Contrary to most organisms in which three enzymes compose the 2-oxoglutarate dehydrogenase complex (ODH), actinobacteria rely on a two-in-one protein (OdhA) in which both the oxidative decarboxylation and succinyl transferase steps are carried out by the same polypeptide. Here we describe high-resolution cryo-EM and crystallographic snapshots of representative enzymes from Mycobacterium smegmatis and Corynebacterium glutamicum, showing that OdhA is an 800-kDa homohexamer that assembles into a three-blade propeller shape. The obligate trimeric and dimeric states of the acyltransferase and dehydrogenase domains, respectively, are critical for maintaining the overall assembly, where both domains interact via subtle readjustments of their interfaces. Schematic illustration of the reaction steps involved in the oxidative decarboxylation of 2-oxoglutarate with generation of succinyl-CoA and NADH/H+ (ODH reaction), with emphasis on the catalytic steps catalyzed by OdhA. These include the ThDP-dependent decarboxylation of the 2-oxoglutarate substrate followed the reductive acylation of the lipoyl group provided by E2p (both catalyzed by the OdhA E1o domain), and the transfer of the succinyl moiety to the CoASH acceptor (catalyzed by the OdhA E2o domain).

Therefore, based on the MsKGD structure and on secondary structure predictions, we produced a truncated version of OdhA deprived of the flexible N-terminal segment (OdhAΔ97), which produced crystals diffracting up to 2.5 Å resolution. The single protomer shows the presence of an N-terminal acyltransferase (E2o) domain, spanning from the construct N-terminus to residue Asn349, connected by a 17-residue linker to the C-terminal, ThDP-dependent oxoglutarate dehydrogenase domain (E1o). In addition, a ThDP-Mg2+ cofactor is bound at the E1o domain dimeric interface, in an equivalent pose and active site environment as in the M. smegmatis E1o (MsKGDΔ360) high-resolution crystal structures. On the other hand, the E2o N-terminal domain shows the known, compact triangular trimeric conformation of the chloramphenicol acetyltransferase (CAT) family, characterized by an N-terminal β-strand that protrudes to make a strand exchange (mixed β-sheet) with the neighboring monomer. Furthermore, despite the overall conservation of the CAT fold, a notable difference between the OdhA succinyltransferase domain and other E2o domains resides in the β-harpin that normally lies close to the three-fold axis and is located on the inside surface of the cubic assembly, here replaced by a short α-helix (connected by flexible linkers) spanning residues 296-302.

> GKLPEPGQTPIRGIFKSIAKNMDISLEIPTATSVRDMPARLMFENRAMVNDQLKRTRGGKISFTHIIGYAMVKAVMAHPDMNNSYDVIDGKPTLIVPEHINLGLAIDLPQKDGSRALVVAAIKETEKMNFSEFLAAYEDIVARSRKGKLTMDDYQGVTVSLTNPGGIGTRHSVPRLTKGQGTIIGVGSMDYPAEFQGASEDRLAELGVGKLVTITSTYDHRVIQGAVSGEFLRTMSRLLTDDSFWDEIFDAMNVPYTPMRWAQDVPNTGVDKNTRVMQLIEAYRSRGHLIADTNPLSWVQPGMPVPDHRDLDIETHNLTIWDLDRTFNVGGFGGKETMTLREVLSRLRAAYTLKVGSEYTHILDRDERTWLQDRLEAGMPKPTQAEQKYILQKLNAAEAFENFLQTKYVGQKRFSLEGAEALIPLMDSAIDTAAGQGLDEVVIGMPHRGRLNVLFNIVGKPLASIFNEFEGQMEQGQIGGSGDVKYHLGSEGQHLQMFGDGEIKVSLTANPSHLEAVNPVMEGIVRAKQDYLDKGVDGKTVVPLLLHGDAAFAGLGIVPETINLAKLRGYDVGGTIHIVVNNQIGFTTTPDSSRSMHYATDYAKAFGCPVFHVNGDDPEAVVWVGQLATEYRRRFGKDVFIDLVCYRLRGHNEADDPSMTQPKMYELITGRETVRAQYTEDLLGRGDLSNEDAEAVVRDFHDQMESVFNEVKEGGKKQAEAQTGITGSQKLPHGLETNISREELLELGQAFANTPEGFNYHPRVAPVAKKRVSSVTEGGIDWAWGELLAFGSLANSGRLVRLAGEDSRRGTFTQRHAVAIDPATAEEFNPLHELAQSKGNNGKFLVYNSALTEYAGMGFEYGYSVGNEDSIVAWEAQFGDFANGAQTIIDEYVSSGEAKWGQTSKLILLLPHGYEGQGPDHSSARIERFLQLCAEGSMTVAQPSTPANHFHLLRRHALSDLKRPLVIFTPKSMLRNKAAASAPEDFTEVTKFQSVINDPNVADAAKVKKVMLVSGKLYYELAKRKEKDGRDDIAIVRIEMLHPIPFNRISEALAGYPNAEEVLFVQDEPANQGPWPFYQEHLPELIPNMPKMRRVSRRAQSSTATGVAKVHQLEEKQLIDEAFEA>MFKHTRKLQYNAKPDRSDPIMARRLQESLGGQWGETTGMMSFLSQGWASTGAEKYKDLLLDTGTEEMAHVEMISTMIGYLLEDAPFGPEDLKR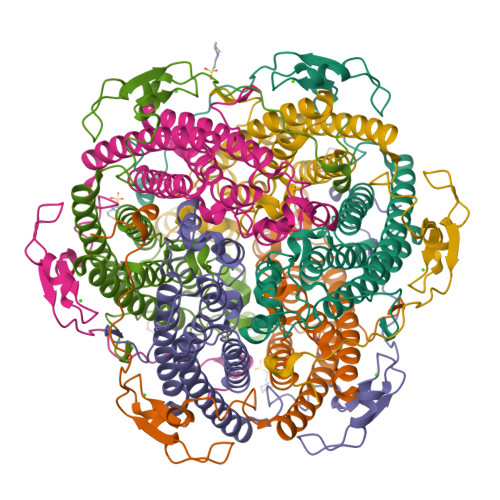DPSLATTMAGMDPEHSLVHGLNASLNNPNGAAWNAGYVTSSGNLVADMRFNVVRESEARLQVSRLYSMTEDEGVRDMLKFLLARETQHQLQFMKAQEELEEKYGIIVPGDMKEIEHSEFSHVLMNFSDGDGSKAFEGQVAKDGEKFTYQENPEAMGGIPHIKPGDPRLHNHQG[6x]> MFHSSAMVNSHRKPMFNIHRGFYCLTAILPQICICSQFSVPSSYHFTEDPGAFPVATNGERFPWQELRLPSVVIPLHYDLFVHPNLTSLDFVASEKIEVLVSNATQFIILHSKDLEITNATLQSEEDSRYMKPGKELKVLSYPAHEQIALLVPEKLTPHLKYYVAMDFQAKLGDGFEGFYKSTYRTLGGETRILAVTDFEPTQARMAFPCFDEPLFKANFSIKIRRESRHIALSNMPKVKTIELEGGLLEDHFETTVKMSTYLVAYIVCDFHSLSGFTSSGVKVSIYASPDKRN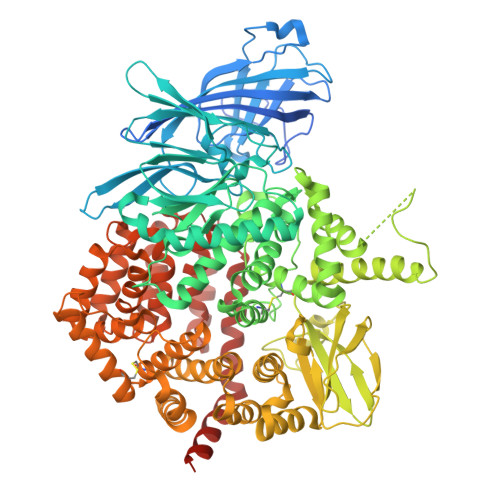QTHYALQASLKLLDFYEKYFDIYYPLSKLDLIAIPDFAPGAMENWGLITYRETSLLFDPKTSSASDKLWVTRVIAHELAHQWFGNLVTMEWWNDIWLKEGFAKYMELIAVNATYPELQFDDYFLNVCFEVITKDSLNSSRPISKPAETPTQIQEMFDEVSYNKGACILNMLKDFLGEEKFQKGIIQYLKKFSYRNAKNDDLWSSLSNSCLESDFTSGGVCHSDPKMTSNMLAFLGENAEVKEMMTTWTLQKGIPLLVVKQDGCSLRLQQERFLQGVFQEDPEWRALQERYLWHIPLTYSTSSSNVIHRHILKSKTDTLDLPEKTSWVKFNVDSNGYYIVHYEGHGWDQLITQLNQNHTLLRPKDRVGLIHDVFQLVGAGRLTLDKALDMTYYLQHETSSPALLEGLSYLESFYHMMDRRNISDISENLKRYLLQYFKPVIDRQSWSDKGSVWDRMLRSALLKLACDLNHAPCIQKAAELFSQWMESSGKLNIPTDVLKIVYSVGAQTTAGWNYLLEQYELSMSSAEQNKILYALSTSKHQEKLLKLIELGMEGKVIKTQNLAALLHAIARRPKGQQLAWDFVRENWTHLLKKFDLGSYDIRMIISGTTAHFSSKDKLQEVKLFFESLEAQGSHLDIFQTVLETITKNIKWLEKNLPTLRTWLMVNTRHHHHHH> DYPKPSTRPPRHN;> CNWTGVKCNRRGEVSEIQLKEKQLQGSLPVTSLRSLKSLTSLTLSSLQLTGVIPKEIGDFTELELL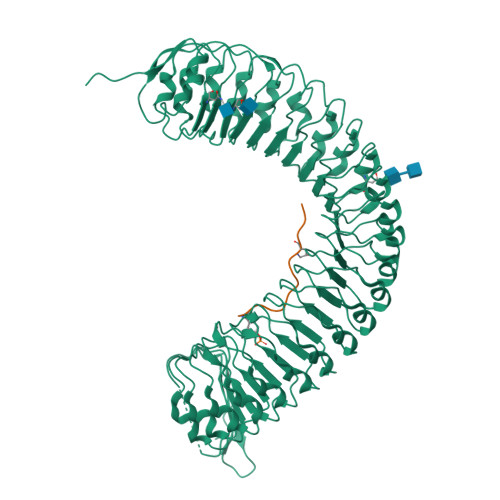DLSDNSLSGDIPVEIFRLKKLKTLSLNTNNLEGHIPMEIGNLSGLVELMLFDNKLSGEIPRSIGELKNLQVLRAGGNKNLRGELPWEIGNCENLVMLGLAETSLSGKLPASIGNLKRVQTIAIYTSLLSGPIPDEIGYCTELQNLYLYQNSISGSIPTTIGGLKKLQSLLLWQNNLVGKIPTELGNCPELWLIDFSENLLTGTIPRSFGKLENLQELQLSVNQISGTIPEELTNCTKLTHLEIDNNLITGEIPSLMSNLRSLTMFFAWQNKLTGNIPQSLSQCRELQAIDLSYNSLSGSIPKEIFGLRNLTKLLLLSNDLSGFIPPDIGNCTNLYRLRLNGNRLAGSIPSEIGNLKNLNFVDISENRLVGSIPPAISGCESLEFLDLHTNSLSGSLLGTTLPKSLKFIDFSDNALSSTLPPGIGLLTELTKLNLAKNRLSGEIPREISTCRSLQLLNLGENDFSGEIPDELGQIPSLAISLNLSCNRFVGEIPSRFSDLKNLGVLDVSHNQLTGNLNVLTDLQNLVSLNISYNDFSGDLPNTPFFRRLPLSDLASNRGLYISNAIST>ENYGIEWHSVRDSEGQKLLIGVGPEGISICKDDFSPINRIAYPVVQMATQSGKNVYLTVTKESGNSIVLLFKMISTRAASGLYRAITETHAFYRCDTVTSA[3x]

The second pathway involves the sterol-regulated inducible degrader of the LDLR (IDOL, also known as MYLIP), which is an E3 ubiquitin ligase that promotes the ubiquitylation and subsequent lysosomal degradation of the LDLR. Two distinct protein domains are present in IDOL: an N-terminal FERM (band 4.1/ezrin/radixin/moesin) and a C-terminal RING domain. In contrast to secreted PCSK9, which interacts with the LDLR extracellularly, IDOL is a 45-kDa cytoplasmic protein that interacts with the intracellular tail of the LDLR via its FERM domain. Here we present two crystal structures of the FERM domain of human IDOL.

We obtained diffracting crystals for two different constructs: IDOL FERM domain, which spans residues 1–344 (FERM344), and the third lobe of the FERM domain, F3ab (residues 183–283). The F3ab subdomain crystallized in space group P212121, with cell dimensions a = 56.37 Å, b = 69.54 Å, c = 74.32 Å, α = β = γ = 90°, with three subunits in the asymmetric unit and a solvent content of 43%. The F3ab conformation is well-conserved between the FERM344 and the three copies in the asymmetric unit of the F3ab crystal structure. Moreover, there are clear differences in the F3c′ region, where the FERM344 crystal structure has an α helix (α7), following the F3ab, which spans residues 279–300 and folds back onto the F3ab. This region has lost helical conformation in all three copies of the F3ab structure, and in one case (F3ab monomer B) even the previous helix α6 is partially unraveled. Because the expression construct used to crystallize F3ab has an incomplete F3c′, helix α7 is unfolded and helix α6 is shorter in all of the three F3ab monomer structures. In fact, in two of the three copies in the asymmetric unit, this unraveled region contacts another F3ab molecule, where it takes on the role of the interacting peptide. The unraveled peptide binds in the F3ab peptide-binding site, making an interaction that closely resembles the β-β association observed in many FERM-substrate peptide complexes. This confirms that the F3ab subunit is intrinsically capable of forming the peptide interaction observed in other FERM receptor interactions.>SNAMGTKNIGKGLTFEDILLVPNYSEVLPREVSLETKLTKNVSLKIPLISSAMDTVTEHLMAVGMARLGGIGIIHKNMDMESQVNEVLKVKNSGGLRVGAAIGVNEIERAKLLVEAGVDVIVLDSAHGHSLNIIRTLKEIKSKMNIDVIVGNVVTEEATKELIENGADGIKVGIGPGSICTTRIVAGVGVPQITAIEKCSSVASKFGIPIIADGGIRYSGDIGKALAVGASSVMIGSILAGTEESPGEKELIGDTVYKYYRGMGSVGAMKSGSGDRYFQEKRPENKMVPEGIEGRVKYKGEME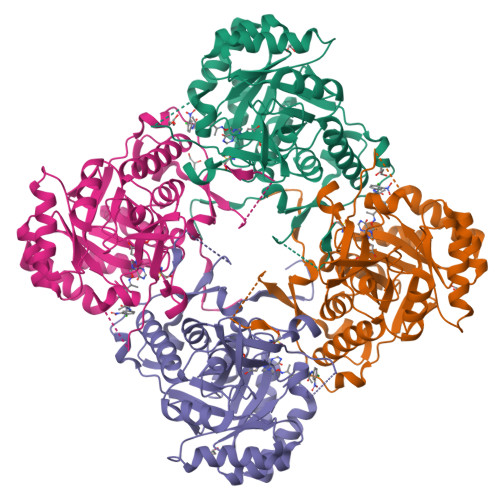GVVYQLVGGLRSCMGYLGSASIEELWKKSSYVEITTSGLRESHVHDVEIVKEVMNYSK[4x]>MPNILYKIDNQYPYFTKNEKKIAQFILNYPHKVVNMTSQEIANQLETSSTSIIRLSKKVTPGGFNELKTRLSKFLPKEVTQYNVELVDNESTISLKNK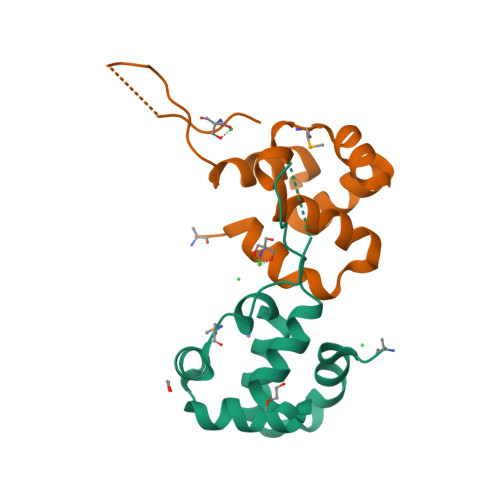LHSRSKAAL[2x]> SNAALNAAQEKEVRALVRDTLVSNPEILEEAIMALQTKKADEQQAQFRQALASEHDALYNDAASPRIGAKDAKLV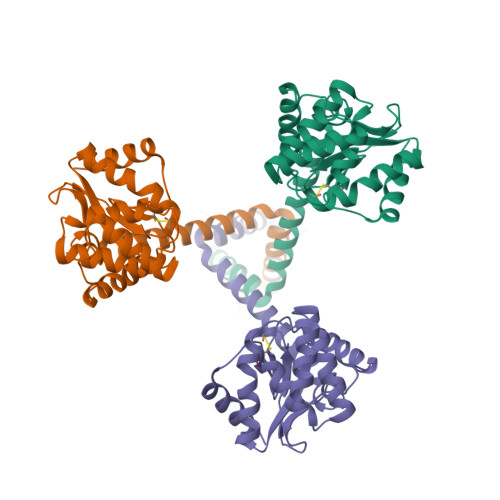LVSFTDYNCPYCKRFDPLLEKITEQYPDVAVIIKPLPFKGESSAKASQAVLSVWKEDPKAFLALHQRLMQKKTMLDNASIEDAMKSTNTSKIKLTDDSLKTLQNNLELSRKLGIQGTPATVIGDTILPGAVDYDQLEIIVKEQLAKVKK>TVETKELNQPLDVVVLLDNSNSMNNERANNSQRALKAGEAVEKLIDKITSNKDNRVALVTYASTIFDGTEATVSKGVADQNGKALNDSVSWDYHKTTFTATTHNYSYLNLTNDANEVNILKSRIPKEAEHINGDRTLYQFGATFTQKALMKANEILETQSSNARKKLIFHVTDGVPTMSYAINFNPYISTSYQNQFNSFLNKIPDRSGILQEDFIINGDDYQIVKGDGESFKLFSDRKVPVTGGTTQAAYRVPQNQLSVMSNEGYAINSGYIYLYWRDYNWVYPFDPKTKKVSATKQIKTHGEPTTLYFNGNIRPKGYDIFTVGIGVNGDPGATPLEAEKFMQSIS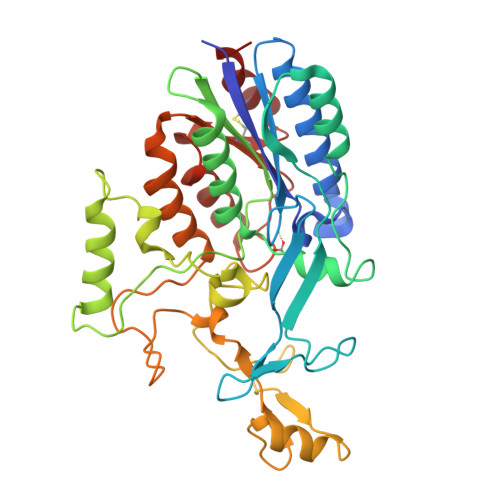SKTENYCNVDDTNCIYDELNKYFK[4x]> E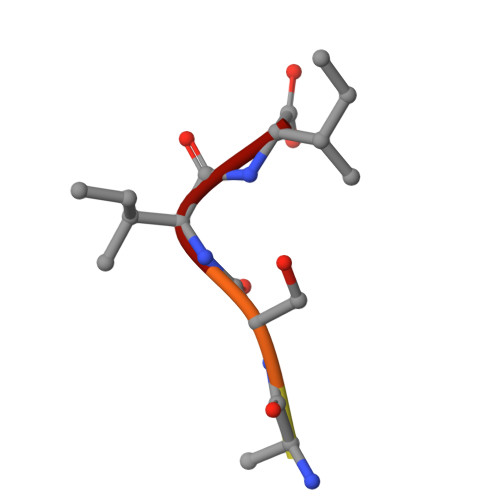VTSII>GASTERVLRAGRQLHRHLLATCPNLIRDRKYHLRLYRQCCSGRELVDGILALGLGVHSRSQVVGICQVLLDEGALCHVKHDWAFQDRDAQFYRFPGPEPEPVGTHEMEEELAEAVALLSQRGPDALLTVALRKPPGQRTDEELDLIFEELLHIKAVAHLSNSVKRELAAVLLFEPHSKAGTVLFSQGDKGTSWYIIWKGSVNVVTHGKGLVTTLHEGDDFGQLALVNDAPRAATIILREDNCHFLRVDKQDFNRIIKDVEAKTMRLEEHG[2x]

EPAC1, a cAMP-activated GEF for Rap GTPases, is a major transducer of cAMP signaling and a therapeutic target in cardiac diseases. Another major transducer of cAMP signaling is the EPAC protein family, comprised of EPAC1 and EPAC2. EPAC1 has the same domain organization as EPAC2, apart from the replacement of the first CNB domain by a 50-residue domain without recognizable structural homology, suggesting that its mechanism of autoinhibition release shares common features with that of EPAC2. We find that anionic membranes activate EPAC1 independently of cAMP, increase its affinity for cAMP by two orders of magnitude, and synergize with cAMP to yield maximal GEF activity.

The structure shows that the DEP and CNB domains are connected by a kinked helix (residues 154–181, with the kink located at P171), which is sandwiched between the two domains and entirely mediates their interaction. We note a single difference between EPAC1 and EPAC2, located at Gln 270 in EPAC1, which forms a hydrogen bond with the sugar hydroxyl of cAMP that is not seen with the equivalent Lys 405 in EPAC2. The potential to form hydrogen bonds at this residue likely contributes to the distinct selectivities of EPAC1 and EPAC2 for cAMP-derived agonists. The structure confirms that it lacks a positively charged pocket that could accommodate PS or PIP2 headgroups, such as the phosphoinositide-binding pocket of PH domains. Combining our EPAC1DEP-CNB structure to a model of EPAC1CNB-GEF/Rap1, we then built a composite model of cAMP-activated EPAC1DEP-CNB-GEF bound to Rap1 and used it to examine how EPAC1 binds to anionic membranes. We identified an extended cationic tract at the surface in the EPAC1DEP-CNB-GEF model, comprised of the polybasic loop in the DEP domain (residues 75RDRKYHLRLYRQ86), and numerous lysines and arginines in the CNB and GEF domains.> MPEQSNDYRVAVFGAGGVGKSSLVLRFVKGTFRESYIPTVEDTYRQVISCDKSICTLQITDSKSGDGNRALQRHVIARGHAFILVYSITSRQSL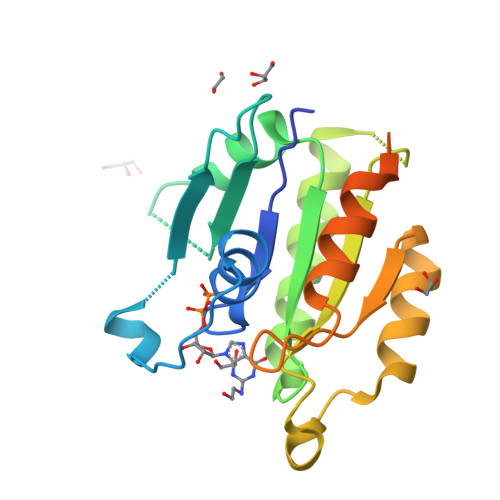EELKPIYEQICEIKGDVESIPIMLVGNKCDESPSREVQSSEAEALARTWKCAFMETSAKLNHNVKELFQELLNLEKRRTVSLQIDGKKSKQQKRKEKLKGKCVIM> MGPVQVNSDLKLLFSNNGAAASSNQIYMNMKLQNTGSSTYDLSKITIRYFYTSDDDKALTYYSDYVSIGSASATFNNLSPVHAKANKYIEIKLASGTLGA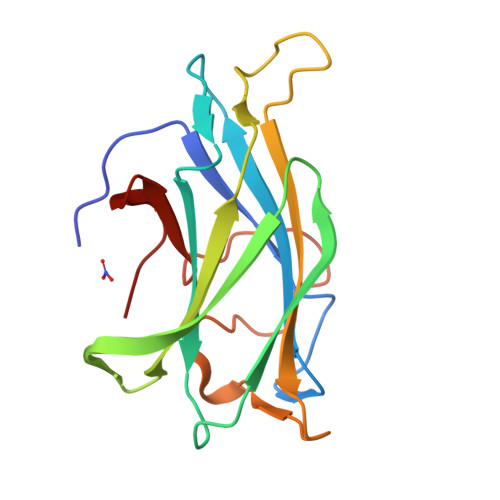AGAQWPSQSEVTIQGRVAKADWTNVDQSNDYSYPGSMSQFGENKLVAVYYNGALVYGTPP>MDKYNNYSNVIKNKSSISPLLAAAAKIEPEITVLSSASKSNRSQYSQSLADTLLGLGYRSIFDIAKVSRQRFIKRHDESLLGNGAVIFDKAVSMANQVLQKYRKNRLEKSNSPLVPQTSSSTDASSESQTNKLPEYNQLFPEPWDNFCRPGAIEALDSPASYLLDLYKFIQSVELDGSNQARKLETRRADIPKLSLDNDALYKEVTALSIVNDVLSGSAREYIDQSGQADKAVNQILGDTHFPFTLPYSLPTQQINKGLGASNIELGTVIQRVDPQFSWNTTQEKYNQVLLAYTQLSSEQIALLSLPDVFTQNFLTQTELSAGYLSASTTEILAEKDLSRHGYIVKAADNIKGPTQLVEHSDASYDVIELTCTNQAKETITVKLRGENIITYQRTKARMVPFDNSSPFSRQLKLTFVAEDNPSLGNLDKGPYFANMDIYAAEWVRENVSSETMVSRPFLTMTYRIAIAKAGASLEELQPEADAFFINNFGLSAEDSSQLVKLVAFGDQTGSKAEEIESLLSCGENLPIVSPNVIFANPIFGSYFNDEPFPAPYHFGGVYINAHQRNAMTIIRAEGGREIQSLSNFRLERLNRFIRLQRWLDLPSHQLDLLLTSVMQADADNSQQEITEPVLKSLGLFRHLNLQYKITPEIFSSWLYQLTPFAVSGEIAFFDRIFNREQLFDQPFILDGGSFTYLDAKGSDAKSVKQLCAGLNISAVTFQFIAPLVQSALGLEAGTLVRSFEVVSSLYRLVSIPQTFGLSTEDGLILMNILTDEMGYLAKQPAFDDKQTQDKDFLSIILKMEALSAWLTKNNLTPASLALLLGVTRLAVVPTNNMVTFFKGIANGLSENVCLTTDDFQRQELEGADWWTLLSTNQVIDDMGLVLDIHPVWGKSDEEMLMEKIQSIGVSNDNNTLSIIVQILIQAKNAQENLLSQTISAEYGVERSVVPLQLRWLGSNVYSVLNQVLNNTPTDISSIVPKLSELTYSLLIYTQLINSLKLNKEFIFLRLTQPNWLGLTQPKLSTQLSLPEIYLITCYQDWVVNANKNEDSIHEYLEFANIKKTEAEKTLVDNSEKCAELLAEILAWDAGEILKAASLLGLNPPQATNVFEIDWIRRLQTLSEKTMISTEYLWQMGDLTENSEFSLKEGVGEAVMAALKAQGDSDNV[5x];>[5x]MSNSIEAKLQEDLRDALVDYYLGQIVPNSKDFTNLRSTIKNVDDLYDHLLLDTQVSAKVITSRLSLVTQSVQQYINRIALNLEPGLSINQQEATDWEEFANRYGYWAANQQLRMFPEIYVDPTLRLTKTEFFFQLESALNQGKLTDDVAQKAVLGYLNNFEEVSNLEIIAGYQDGIDIENDKTYFVARTRMQPYRYFWRSLDASQRNANSQELYPTAWSEWKAISVPLENVANGIVRPIMMDNRLYISWFEVAEEKETDSDGNIIVSGRYRTKIRLAHLGFDGVWSSGTTLREEVLADQMEEMIAVVDRMEDEPRLALVAFKEMSESWDVVFSYICDSMLIESSNLPTTTHPPKPGDGDKGLSDLDDYGANLVWFYLHETANGGKAEYKQLILYPVIINRDWPIELDKTHQGDFGTVDDFTLNSNYTGDELSLYLQSSSTYKYDFSKSKNIIYGIWKEDANNNRCWLNYKLLTPEDYEPQINATLVMCDKGDVNIITGFSLPNGGVDAGGKIKVTLRVGKKLRDKFQIKQFSQTQYLQFPEASSADVWYIGKQIRLNTLFAKELIGKASRSLDLVLSWETQNSRLEEAILGGAAELIDLDGANGIYFWELFFHMPFMVSWRFNVEQRYEDANRWVKYLFNPFECEDEPALLLGKPPYWNSRPLVDEPFKGYSLTQPSDPDAIAASDPIHYRKAVFNFLTKNIIDQGDMEYRKLQPSARTLARLSYSTASSLLGRRPDVQLTSFWQPLTLEDASYKTDSEIRAIEMQSQPLTFEPVVHDQTMSAVDNDIFMYPMNNELRGLWDRIENRIYNLRHNLTLDGKEINMDLYDSSISPRGLMKQRYQRVVTARNASKMNFKVPNYRFEPMLNRSKSGVETLIQFGSTLLSLLERKDSLSFDAYQMIQSGDLYRFSIDLQQQDIDINKASLEALQVSKQSAQDRYDHFKELYDENISSTEQKVIELQSQAANSLLMAQGMRTAAAALDVIPNIYGLAVGGSHWGAPLNAAAEIIMIKYQADSSKSESLSVSESYRRRRQEWELQYKQAEWEVNSVEQQINLQNMQIKAANKRLEQVEAQQQQAMALLDYFSERFTNESLYTWLISQLSSLYLQAYDAVLSLCLSAEASLLYELNLGEQSFVGGGGWNDLYQGLMAGETLKLALMRMERVYVEQNSRRQEITKTISLKALLGESWPAELNKLKQKTPINFNLEEQIFVEDYQELYQRRIKSVSVSLPMLVGPYEDVCAQLTQTSSSYSTRADLKTVENMLTKRTFADTPHLVRSIQPNQQISLSTGVNDSGLFMLNFDDERFLPFEGSGVDSSWRLQFTNLKQNLDSLNDVILHVKYTAAIGSSTFSQGVRKILANINNDE;>[5x]MVNKYTYTSSKAMSDISDVIGEPLAAWDSQVGGRVFNVIFDGKVYTNTYWVERWQVPGIGSSDGNPHNAWKFVRAATADEINKIGNPTTADVKPTENIPSPILVEDKYTEETYSRPDVNFKEDGSQGNLSYTATRVCAPMYNHYVGDKTKPKLSAYITDWCQYDARLDGGGSKEEERGRGFDLATLMQNPATYDRLIFSFLGICGDIGNKSKKVQEVWDGWNAQAPSLGLPQIGKGHIVPLDPYGDLGTARNVGLPPESADTSIESGTFLPYYQQNRAAGLLGGLRELQKKAHAMGHKLDLAFSIGGWSLSSYFSALAENPDERRVFVASVVDFFVRFPMFSCVDIDWEYPGGGGDEGNISSDKDGENYVLLIKELRSALDSRFGYSNRKEISIACSGVKAKLKKSNIDQLVANGLDNIYLMSYDFFGTIWADYIGHHTNLYSPKDPGEQELFDLSAEAAIDYLHNELGIPMEKIHLGYANYGRSAVGGDLTTRQYTKNGPALGTMENGAPEFFDIVKNYMDAEHSLSMGKNGFVLMTDTNADADFLFSEAKGHFISLDTPRTVKQKGEYAAKNKLGGVFSWSGDQDCGLLANAAREGLGYVADSNQETIDMGPLYNPGKEIYLKSISEIKSK;> MQNSQEMAITTLSLPKGGGAINGMGESVGQAGPDGMVTFSIPLPFSAGRGVAPALSLSYSSGAGNGPFGMGWQCSAMSISRRTQKGVPQYNEDDEFLSPSGEVMAIALNDSGFEDVRTANRLQGIPLPFSYKVTRYQPRLIQDFIKIEYWQPVKQTDGTPFWIIYSPDGQTHILGKNSHSRVANAENPSQIASWLLEETVTPTGEHIYYQYSGENQVNCTDAEIALHPQDSAQRYLARIDYGNISPQASLFVLDEELPNLTQWLFHLVFDYGERDISINKIPTFEGGTTGWLARPDMFSRYDFGIEIRNRRLCHQVLGFHRLEALNDRDVTDEIPVLVNRLTLDYDLNNSVSTLVAVRQVAYETDGSPITQPPLEFDYQRFDTGSIPGWQEMPQLEAFNGYQPYQMIDLYGEGTPGILYQETPGAWWYKSPQRQIGGDSNAVTYGAMKALPKIPRLQEGATLMDINGDGRLDWVITSAGVRGFHSIHSTGEWTHFTPLNTLPTEYFHPKAQLADLVGAGLSDLVLIGPKSVRLYANQQGNWAPAQDVTQAENVSLPVIGIDSRQLVAFADMLGSGQQHLVEITADSVKCWPNMGHGRFGQPLTLEGFSQPQTSFNPDRVFLADIDGSGTNDIIYAHSECLEIYLNESGNRFSKPISLLLPDGVNFDNTCQLQAADIQGLGIASLVMTVPHMSPTHWRCDLALNKPWLLNVMNNNRGAETCLFYRSSAQFWLDEKQLVEAAGQQPECHLPFPMHLHWRSEIFDEITGNRLTQEQEYAHGSWDGQEREFRGFGRLIQRDTDGFAQGTVDIPTHPSRTVSWFATGIPEIDTTLSAEFWRGDDQAFSPFSPRFTRWENDSEAGSDVAFIPSEHDAFWLNRAMKGQLLRSELYGDDGTPEAEIPYSVTEMRHQVRALPTTDATVPSAWCSTIETRSYQYQRVAADPQCSQQVVIKADRYGSPLLSVAINYPRRKKPEKSPY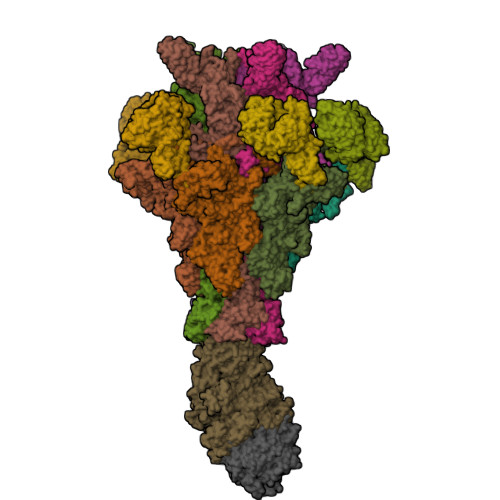PDDLPETLFDSSYDTQQQQLHLTKQQQNYFHLTNDDNWLLGLPKEQRNDGYQYDQERAPANGFTLETLIASNSLIGSNQPFTYLGQSRVAYQGGVDEQPSLQALVAYGETAILDEKTLQAFVGVLDSKTRDELLFSAGYQLAPRLFRVESEPDVWVARQGYSEFGDYSQFWRPLSQRSTLLTGKTTLKWDKHYCVVIETQDAAQLVTQARYDYRFLTPYSLTDANDNQHYVVLNPFGEVIASRFWGTEAGKDAGYSTPQAKPFVVPATIEAALALSPGIPVAHCAIFEPESWMQKLTQHDVSERMADNGTLWNALLQARFVTEDGYVCALGRRRWMARHGLSVLMLTLLAEIPRTPPHSLTITTDRYDSDDQQQLRQRILFSDGFGRLLQSAQRVEAGESWQRSEDSSLVVNVSGTPALVVTDNRWAVSGRTEYDGKGQGIRVYQPYFLDDWRYLSDDSARTDLFADTHIYDPLGREYQVITAKGYRRERQYTPWFVVNQDENDTAANLAI;> MDIQLFSKTPSVTVFDNRGLSVRDIAYRRHPDTPKVTEECITYHQFDFRGFLAQSLDPRLNHKEVTNFSYLTDLNGNIIYTQSVDAGNTLVLNDTEGRSVIAMTNISRGENGKDDLSLAVTRTFQYENAPLPGRPLSVTEQVNGENARITEHFVYAGNTPQEKNLNLAGQCVSYYDAAGLIQTDSVSLTGKPLSVSRKLLKNLDDTNILADWQGNDTSAWNSLLATEIYTTVTRTDAAGAVLTTIDAVGNQQRVAFDIAGQLSASWLTLKGGQEQVIIKVLTYSAAGQKLREEGGNGVVTTYTYEAETQRLIGIKTERPNGHAAGAKVLQDLRYEYDPVGNVLSITNDAEETRFWRNQKVVPENAYRYDSLYQLVSASGREVAGAGQQGSDLPSPLVPLPSDSSVYTNYTRTYTYDSAGNLMRIRHSAPATNNNYTLNITVSERSNRGVMSSLTENPADVDALFTASGSQKCLQQGQSLIWTPRGELRTVLLVARGETADDSESYRYDGSSQRILKISSQQTNHSARVQRALYLPGLEWRTMTGGVAEAENLQVICIGEAGRAQVRVLHWESGKPDGIINDQIRWSYDNLTCSSGLEVDGDGLVISMEEYYPYGGTAVWAARSHIETAYKTVRYSGKERDATGLYYYGFRYYQPWAGRWLSADPAGTVDGLNLYRMVRNNPLRLTDPDGMAPLDWLDLDTTNASRDIVKAIYQLNQIDGPHRGVRDTYQRMTESTGMILQETLNNEAVLKGIKQKDKEKKSRGMKFTNSKLKTYAAHAGVLNTLQPDPVYKDGFLNLPGSLGNKNTFPGVELIEDKVKPSLSQYHPDKLGKSQRWKPESSLGYYRVADTEAFITGIRSQYKSSGTDLHAVVEGRIRDHLLANNNVLPKMAGIAGLHAEVQALNYIISNPDIEGGNAERLNGSYIFTQRLVGDVNQDFPACYNCSGIISGLENVMTGRVNNDVRLKRRKSF> PPGVDCPMEFWTKEENQSVVVDFLLPTGVYLNFPVSRNANLSTIKQLLWHRAQYEPLFHMLSGPEAYVFTCINQTAEQQELEDEQRRLCDVQPFLPVLRLVAREGDRVKKLINSQISLLIGKGLHEFDSLCDPEVNDFRAKMCQFCEEAAARRQQLGWEAWLQYSFPLQLEPSAQTWGPGTLRLPNRALLVNVKFEGSEESFTFQVSTKDVPLALMACALRKKATVFRQPLVEQPEDYTLQVNGRHEYLYGSYPLCQFQYICSCLHSGLTPHLTMVHSSSILAMRDEQSNPAPQVQKPRAKPPPIPAKKPSSVSLWSLEQPFRIELIQGSKVNADERMKLVVQAGLFHGNEMLCKTVSSSEVSVCSEPVWKQRLEFDINICDLPRMARLCFALYAVIEKAKKARSTKKKSKKADCPIAWANLMLFDYKDQLKTGERCLYMWPSVPDEKGELLNPTGTVRSNPNTDSAAALLICLPEVAPHPVYYPALEKILELGRHSECVHVTEEEQLQLREILERRGSGELYEHEKDLVWKLRHEVQEHFPEALARLLLVTKWNKHEDVAQMLYLLCSWPELPVLSALELLDFSFPDCHVGSFAIKSLRKLTDDELFQYLLQLVQVLKYESYLDCELTKFLLDRALANRKIGHFLFWHLRSEMHVPSVALRFGLILEAYCRGSTHHMKVLMKQGEALSKLKALNDFVKLSSQKTPKPQTKELMHLCMRQEAYLEALSHLQSPLDPSTLLAEVCVEQCTFMDSKMKPLWIMYSNEEAGSGGSVGIIFKNGDDLRQDMLTLQMIQLMDVLWKQEGLDLRMTPYGCLPTGDRTGLIEVVLRSDTIANIQLNKSNMAATAAFNKDALLNWLKSKNPGEALDRAIEEFTLSCAGYCVATYVLGIGDRHSDNIMIRESGQLFHIDFGHFLGNFKTKFGINRERVPFILTYDFVHVIQQGKTNNSEKFERFRGYCERAYTILRRHGLLFLHLFALMRAAGLPELSCSKDIQ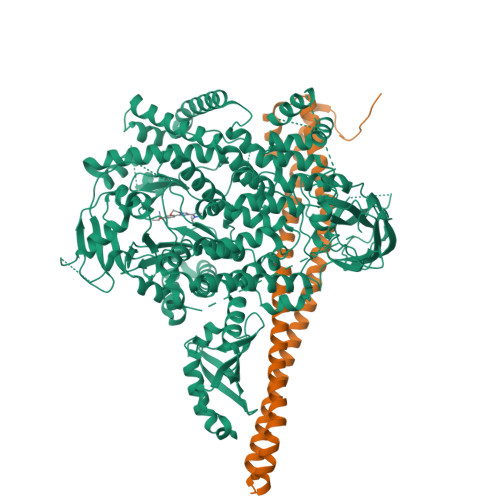YLKDSLALGKTEEEALKHFRVKFNEALRESWKTKVNWLAHNVSKDNRQ;> YQQDQVVKEDNIEAVGKKLHEYNTQFQEKSREYDRLYEDYTRTSQEIQMKRTAIEAFNETIKIFEEQCQTQERYSKEYIEKFKREGNETEIQRIMHNYEKLKSRISEIVDSRRRLEEDLKKQAAEYREIDKRMNSIKPDLIQLRKTRDQYLMWLTQKGVRQKKLNEWLG>SSTPLSPTRITRLQEKEDLQELNDRLAVYIDRVRSLETENAGLRLRITESEEVVDFYFGKLRNIELICQENEGENDPVLQRIV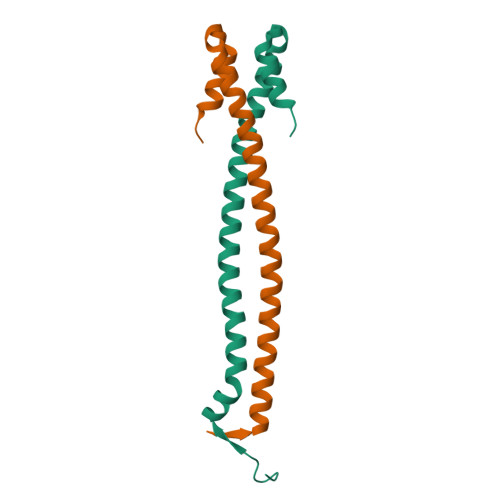DILYATDE[4x]>GSSMGQPGIINNDLQTLLEVKKSLVTNPQEDDPLRQWNSDNINYCSWTGVTCDNTGLFRVIALNLTGLGLTGSISPWFGRFDNLIHLDLSSNNLVGPIPTALSNLTSLESLFLFSNQLTGEIPSQLGSLVNIRSLRIGDNELVGDIPETLGNLVNLQMLALASCRLTGPIPSQLGRLVRVQSLILQDNYLEGPIPAELGNCSDLTVFTAAENMLNGTIPAELGRLENLEILNLANNSLTGEIPSQLGEMSQLQYLSLMANQLQGLIPKSLADLGNLQTLDLSANNLTGEIPEEFWNMSQLLDLVLANNHLSGSLPKSICSNNTNLEQLVLSGTQLSGEIPVELSKCQSLKQLDLSNNSLAGSIPEALFELVELTDLYLHNNTLEGTLSPSISNLTNLQWLVLYHNNLEGKLPKEISALRKLEVLFLYENRFSGEIPQEIGNCTSLKMIDMFGNHFEGEIPPSIGRLKELNLLHLRQNELVGGLPASLGNCHQLNILDLADNQLSGSIPSSFGFLKGLEQLMLYNNSL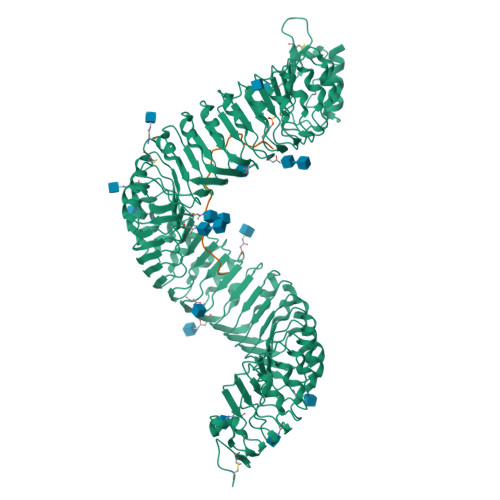QGNLPDSLISLRNLTRINLSHNRLNGTIHPLCGSSSYLSFDVTNNGFEDEIPLELGNSQNLDRLRLGKNQLTGKIPWTLGKIRELSLLDMSSNALTGTIPLQLVLCKKLTHIDLNNNFLSGPIPPWLGKLSQLGELKLSSNQFVESLPTELFNCTKLLVLSLDGNSLNGSIPQEIGNLGALNVLNLDKNQFSGSLPQAMGKLSKLYELRLSRNSLTGEIPVEIGQLQDLQSALDLSYNNFTGDIPSTIGTLSKLETLDLSHNQLTGEVPGSVGDMKSLGYLNVSFNNLGGKLKKQFSRWPADSFLGNTGLCGSPLSRCNRVRSNNKQQGLENLYFQ[2x];>DYGHSSPKPKLVRPPFKLIPN[2x]> MAELISKEGNKVEFKVSVPAAEVNRAYDQVWAGLARDVRVPGFRPGKAPRKVIENRVGKGYVESQVRDRLLETHYSQGLRELGL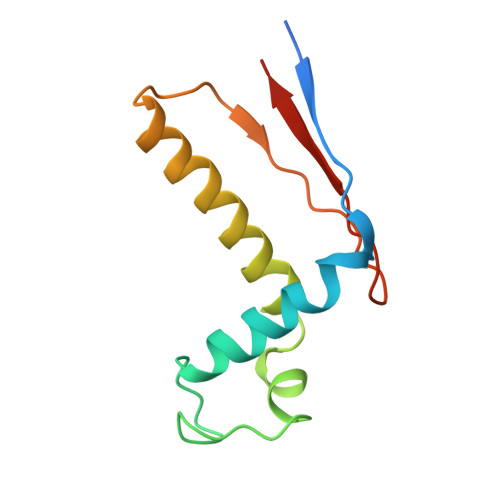NLVDATVDPQDVQSGQAFEFTVKGETYP> GSHMGDQRFGDLVFRQLAPNVWQHTSYLDMPGFGAVASNGLIVRDGGRVLVVDTAWTDDQTAQILNWIKQEINLPVALAVVTHAHQDKMGGMDALHAAGIATYANALSNQLAPQEGMVAAQHSLTFAANGWVEPATAPNFGPLKVFYPGPGHTSDNITVGINGTDIAFGGCLIKDSKAKSLGNLGDADTEHY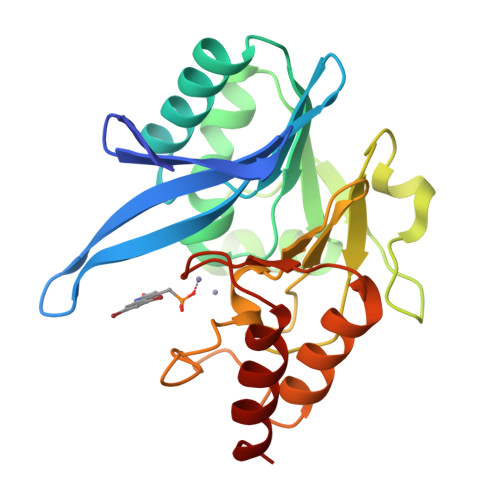AASARAFGAAFPKASMIVMSHSAPDSRAAITHTARMADKLR> MRIGEWMRGLLLCAGLMMCGVVHADISTVPDETYDALKLDRGKATPKETYEALVKRYKDPAHGAGKGTMGDYWEPIAISIYMDPNTFYKPPVSPKEVAERKDCVECHSDETPVWVRAWKRSTHANLDKIRNLKSDDPLYYKKGKLEEVENNLRSMGKLGEKETLKEVGCIDCHVDVNKKDKADHTKDIRMPTADTCGTCHLREFAERESERDTMVWPNGQWPAGRPSHALDYTANIETTVWAAMPQREVAEGCTMCHTNQNKCDNCHTRHEFSAAESRKPEACATCHSGVDHNNWEAYTMSKHGKLAEMNRDKWNWEVRLKDAFSKGGQNAPTCAACHMEYEGEYTHNITRKTRWANYPFVPGIAENITSDWSEARLDSWVLTCTQCHSERFARSYLDLMDKGTLEGLAKYQEA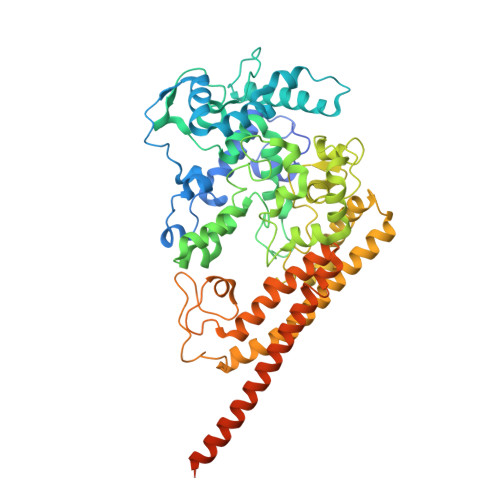NAIVHKMYEDGTLTGQKTNRPNPPEPEKPGFGIFTQLFWSKGNNPASLELKVLEMAENNLAKMHVGLAHVNPGGWTYTEGWGPMNRAYVEIQDEYTKMQELSALQARVNKLEGKQTSLLDLKGTGEKISLGGLGGGMLLAGALALIGWRKRKQTRA BIOTINYL-5-AMP | C20 H28 N7 O9 P S | 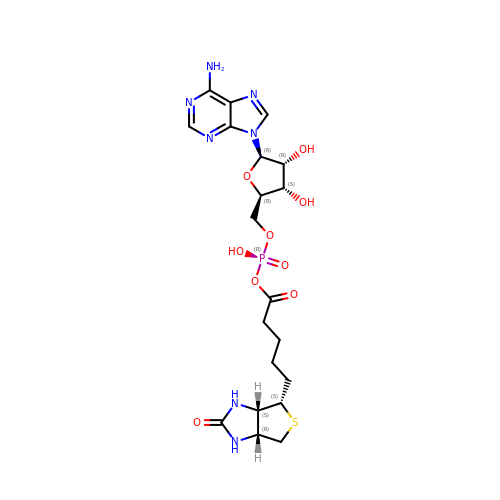UTQCSTJVMLODHM-RHCAYAJFSA-N After transcription, the 3′-end is oligo-uridylylated by a terminal uridylyltransferase, TUT1 (TUTase6)910, one of the members of the non-canonical nucleotidyltransferases. TUT1 is composed of N-terminal Zn-finger, RRM, palm, fingers and KA-1 domains. The C-terminal region of TUT1 is a previously unidentified RNA-binding domain, and it was named the KA-1 domain. Thus, the present structural and biochemical studies have demonstrated that TUT1 acts as a U6 snRNA-specific terminal uridylyltransferase.

Therefore, the amino-terminal putative zinc finger (ZF) and RNA recognition motif (RRM) (amino-acid residues 1–140), the predicted disordered proline-rich region (PRR: amino-acid residues 235–304) and the carboxy-terminal region (amino-acid residues 651–750) neighbouring the nuclear localization signal (NLS) were removed. The truncated TUT1 (TUT1_ΔN) was overexpressed in Escherichia coli, purified and crystallized. The form-I and -II crystals belong to the space groups P21212, and P21, respectively. The data sets were also collected from the apo form-I crystal, and the structure was refined to an R factor of 25.3% (Rfree of 29.7%), using reflections up to 2.8 Å resolution. The TUT1_ΔN structure consists of three domains—catalytic palm (residues 172–403) and fingers (residues 141–171 and 404–598) domains, and an additional distinct domain linked to the C-terminus of the protein (residues 599–874). A comparison between the form-I and -III TUT1_ΔN structures highlights the mobility of the KA-1 domain. The KA-1 domain rotates by ∼40° with respect to the catalytic core domains, using α14 as the axis of rotation.

>MGAAPDSHQLAKALAEAADVGAQMIKLVGLRELSEAERQLRSLVVALMQEVFTEFFPGCVVHPFGSSINSFDVHGCDLDLFLDLGDLEEPQPVPKLPPASPLLEDREEGDLGKASELAETPKEEKAEGAAMLELVGSILRGCVPGVYRVQTVPSARRPVVKFAHRPSGLHGDVSLSNRLALHNSRFLSLASELDGRVRPLVYTLRAWAQGRGLSGSGPLLSNYALTLLVIYFLQTRDPPVLPTVSQLTQKAGEGEQVEVDGWDCSFPRDASRLEPSINVEPLSSLLAQFFSAVSSWDLRGSLLSLREGQALPVAGGLPSNLWEGLRLGPLNLQDPFDLSHNVAANVTSRVAGRLQNCCRAAANYARSLQYQRRSSRGRDWGLLPLLQPSSPSSLLSATPIPLPLAPFTQLTAALVQVFREALGCHIEQATKRTRSEGGGTGQGEAGKGASLPSSASWRCALWHRVWQGRRRARRRLQQQTKEGAGGGAGTRAGWLATEAQVTQELKGLSGGEERPETEPLLSFVASVSPADRMLTVTPLQDPQGLFPDLHHFLQVFLPQAIRHLKLEHHHHHH[2x]> MGAQVSTQKTGAHETSL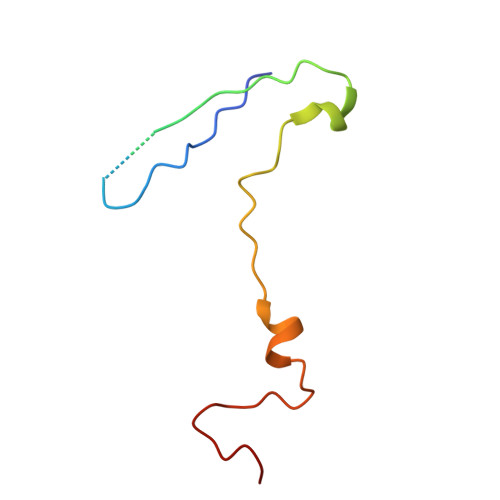SAAGNSVIHYTNINYYKDAASNSANRQDFTQDPGKFTEPVKDIMVKSMPALN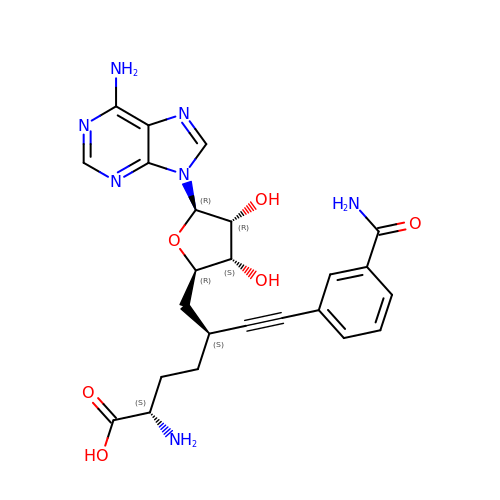9-{9-amino-6-[(3-carbamoylphenyl)ethynyl]-5,6,7,8,9-pentadeoxy-D-glycero-alpha-L-talo-decofuranuronosyl}-9H-purin-6-amine | C24 H27 N7 O6 | QRKSTGPKAQGBDD-GGPTZFPQSA-N> MKLTLWTYEGPPHVGAMRVATAMKDLQLVLHGPQGCTYADLLFTMIERRNARPPVSFSTFEASHMGTDTAILLKDALAAAHARYKPQAMAVALTCTAELLQDDPNGISRALNLPVPVVPLELPSYSRKENYGADETFRALVRALAVPMERTPEVTCNLLGATALGFRHRDDVAEVTKLLATMGIKVNVCAPLGASPDDLRKLGQAHFNVLMYP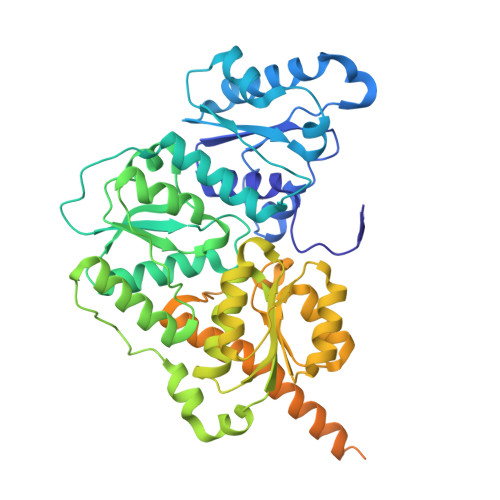ETGESAARHLERACKQPFTKIVPIGVGATRDFLAEVSKITGLPVVTDESTLRQPWWSASVDSTYLTGKRVFIFGDGTHVIAAARIAAKEVGFEVVGMGCYNREMARPLRTAAAEYGLEALITDDYLEVEKAIEAAAPELILGTQMERNIAKKLGLPCAVISAPVHVQDFPARYAPQMGFEGANVLFDTWVHPLVMGLEEHLLTMFREDFEFHDAAGASHHGGKAVAREESPVAPADLAPAATSDTPAAPSPVVVTQASGEIRWMPEAERELRKIPFFVRGKAKRNTELYAAHKGVCDITVETLYEAKAHYAR Flavin-dependent halogenases (FDHs) regioselectively halogenate aromatic substrates using halide ions, O2, and reduced flavin (FADH2) at physiological temperatures in aqueous solution, making them a green alternative to conventional synthetic methods for aryl halide preparation. To better understand mechanistic details that limit FDH catalytic efficiency and potentially hinder their application as in vitro biocatalysts, we investigated the halogenation activity, substrate scope, crystal structures, and ligand binding of the Trp-5-halogenase AbeH and the Trp-6-halogenase BorH. HOCl generation occurs >10 Å away from where the Trp (or other aromatic substrate) binds, and the HOCl must diffuse through a tunnel toward a conserved Lys,29 which either hydrogen bonds with HOCl and positions the Cl for reaction with Trp by EAS25,30,31 or reacts with HOCl to form a chloramine, which in turn transfers Cl to Trp by EAS. Our results show that flavin cosubstrate/coproduct (FADH2/FAD) and substrate (Trp) cannot bind simultaneously to either AbeH or BorH.

Apo-AbeH crystallized in P21 with four molecules in the ASU. There are four AbeH chains in the asymmetric unit, arranged as two dimers (B/D and A/C) with the same dimer interface seen in the AbeH/FAD structure but different crystal packing between the dimers. The monoclinic crystal used to solve the apo-AbeH structure had been soaked in Trp, but there was no electron density in the Trp binding site. The most significant backbone difference between the chains in the apo-AbeH structure and the AbeH/FAD structure is in the flavin binding loop, which is closed over FAD in both chains of the complex structure but is disordered in Chains A and B and in the open conformation in chains C and D in the apo-AbeH structure. In addition, the Gly10-Gly11 peptide bond is flipped, so that in apo-AbeH the Gly10 carbonyl O is hydrogen bonded to the NH of Gly14, and in AbeH/FAD, the Gly11 N–H is engaged in a water-mediated interaction with the FAD pyrophosphoryl group (a similar flip was previously observed between the open and closed conformations of Thal31). In the apo-AbeH structure, all four chains are missing the η3-β9 segment, chains A, C, and D are missing the segment between β16 and β17, and chains C and D are missing five additional residues at the C-terminus. The four apo-AbeH chains have Cα rmsd values ranging from 0.33–0.51 Å with one another and from 0.78–1.11 Å with chain B of the AbeH/FAD structure. In apo-AbeH, even though the flavin binding loop is open/disordered and Glu46 points inward, the gate is closed, and the lid is open. The closed gate explains our inability to soak Trp into this crystal form, but it is unclear why the gate remains closed even though the flavin binding loop is open.

>[4x]PMLKNVVVVGGGTAGWMTASYLTAAFGDRIGVTLVESKRVGSIGVGEATFSTVRHFFEYLGLEEKEWMPACNATYKLAIRFENWREPGHHFYHPFERQRVVDGFPLTDWWLREPRSDRFDKDCFLVGTLCDDLKSPRQLNGELFEGGLGGRSAYRTTLAEQTTQFPYAYHFDATLVANYLRDYAVARGVKHVLDDVQDVALDDRGWISHVVTGESGNLTGDLFIDCTGFRSLLLGKALAEPFQSYQDSLPNDSAVALRVPQDMENRGLRPCTTATAQEAGWIWTIPLFDRIGTGYVYAGDYISPEEAERTLRAFVGPAAEHADANHIKMRIGRSNRHWVNNCVAVGLSSGFVEPLESTGIFFIQHAIEQLVKHFPDERWDDGLRTAYNKLVNNVMDGVREFLVVHYYAAKRQDNQYWKDAKTRPLPDGLAERLERWQTRLPDNESVFPHYHGFESYSYVCMLLGLGGLDLKSSPALGLMDAAPARHEFKLVGEQAAELARTLPTQYEYFAQLHRAR4-[5-[2,6-bis(fluoranyl)phenyl]-2~{H}-pyrazolo[3,4-b]pyridin-3-yl]-2-(4-oxidanylpiperidin-1-yl)-1~{H}-pyrimidin-6-one | C21 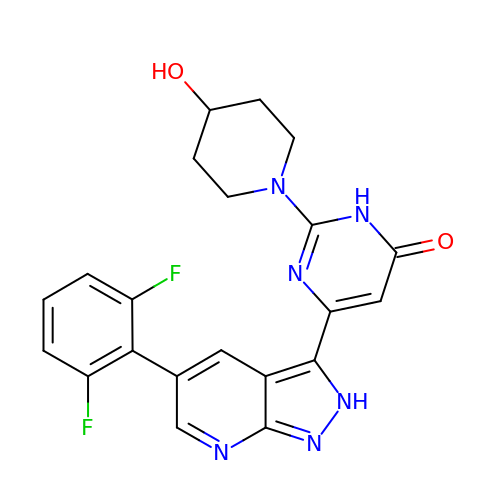H18 F2 N6 O2 | CAASTELLWPCGBG-UHFFFAOYSA-N>MSQTETSHSGYIDFKKESQPSVFQCKKCFQIVGDSNAWVISHREYLSFTLSDAVENSVRVEDTFKRSDDGLCVYSELSCTRCNEVIGKVYNSTPIYLDDIRDMYTFSMDKLQAYQLGNKT[3x]

Mis18 is a key regulator responsible for the centromere localization of the CENP‐A chaperone Scm3 in Schizosaccharomyces pombe and HJURP in humans, which establishes CENP‐A chromatin that defines centromeres. Here, by combining structural, biochemical, and yeast genetic studies, we show that the oligomerization of S. pombe Mis18, mediated via its conserved N‐terminal Yippee‐like domain, is crucial for its centromere localization and function. Amino acid sequence and the predicted secondary structure analysis of Schizosaccharomyces pombe Mis18 suggested the presence of a highly conserved N‐terminal globular domain (residues 1–120; spMis181–120) mainly comprised of β‐strands, followed by a moderately conserved C‐terminal α‐helical domain (residues 121–end; spMis18C‐term‐α). Here, we show that fission yeast Mis18 and its human isoforms, Mis18α and Mis18β, possess two structurally distinct domains: an N‐terminal “Yippee‐like” globular domain and a C‐terminal α‐helical domain.

To structurally characterize spMis181–120, we purified recombinant spMis181–120 as a mono‐disperse sample and obtained crystals that diffracted X‐rays to about 2.6 Å. The structure was determined by single anomalous dispersion (SAD) exploiting the Zn anomalous signal from the bound Zn2+ ions in the crystals. The final model includes amino acid residues 19–118 of spMis181–120. The overall fold of spMis181–120 is formed by antiparallel β‐sheets: a three‐stranded (β1‐β2‐β9: β‐sheet I) and a six‐stranded (β3‐β4‐β8‐β7‐β6‐β5: β‐sheet II) sheet, arranged approximately perpendicular to each other. The two β‐sheets are held together by a Zn2+ ion coordinated via the C‐X‐X‐C motifs from loops L1 and L5. Although these proteins recognize substrates as diverse as nucleic acids to proteins, they do so via a common cradle‐shaped binding pocket formed by β‐sheet II (Fig EV1C and D). The asymmetric unit of the spMis181–120 crystals contained three copies of spMis181–120 assembled in a linear arrangement via two different interfaces (interface I and interface II), resulting in two potential dimeric structures (dimer I and dimer II). While the interface stabilizing dimer I is formed by the stacking of loops L5 and L7 of one monomer over their dimeric counterpart, the dimer II interface is formed by the stacking of β‐sheet I. In contrast, dimer II is stabilized by highly conserved residues (V22, I31, Y114, and L116) and has an extensive binding interface (as compared to dimer I) with a 1,431 Å2 buried surface area. Consistent with this, the other dimer II interface mutants Y114A, Y114E, and V22E also behaved as smaller entities compared to the wild‐type protein when analyzed by native PAGE (Fig EV2B), thus demonstrating that the dimerization of spMis181–120 is mediated via the dimer II interface.>PRPPKVGSSGNASWFQAIKAKKLNSPQPKFEGSGVPDNE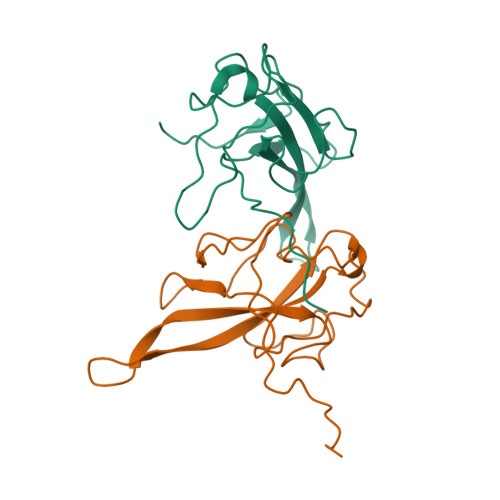NLKTSQQHGYWRRQARFKPGKGRRKPVPDAWYFYYTGTGPAADLNWGDSQDGIVWVAAKGADVKSRSNQGTRDPDKFDQYPLRFSDGGPDGNFRWDFIPL[2x]> GSSMGSQSLYREIHQLISFKDVLPDKNLLPDWSSNKNPCTFDGVTCRDDKVTSIDLSSKPLNVGFSAVSSSLLSLTGLESLFLSNSHINGSVSGFKCSASLTSLDLSRNSLSGPVTTLTSLGSCSGLKFLNVSSNTLDFPGKVSGGLKLNSLEVLDLSANSISGANVVGWVLSDGCGELKHLAISGNKISGDVDVSRCVNLEFLDVSSNNFSTGIPFLGDCSALQHLDISGNKLSGDFSRAISTCTELKLLNISSNQFVGPIPPLPLKSLQYLSLAENKFTGEIPDFLSGACDTLTGLDLSGNHFYGAVPPFFGSCSLLESLALSSNNFSGELPMDTLLKMRGLKVLDLSFNEFSGELPESLTNLSASLLTLDLSSNNFSGPILPNLCQNPKNTLQELYLQNNGFTGKIPPTLSNCSELVSLHLSFNYLSGTIPSSLGSLSKLRDLKLWLNMLEGEIPQELMYVKTLETLILDFNDLTGEIPSGLSNCTNLNWISLSNNRLTGEIPKWIGRLENLAILKLSNNSFSGNIPAELGDCRSLIWLDLNTNLFNGTIPAAMFKQSGKIAANFIAGKRYVYIKNDGMKKECHGAGNLLEFQGIRSEQLNRLSTRNPCNITSRVYEGHTSPTFDNNGSMMFLDMSYNMLSGYIPKEIGSMPYLFILNLGHNDISGSIPDEVGDLRGLNILDLSSNKLDGRIPQAMSALTMLTEIDLSNNNL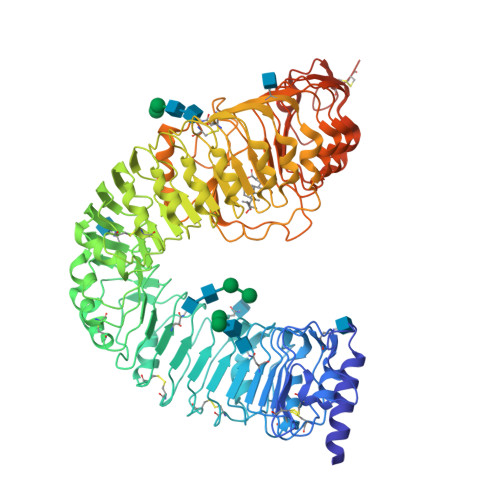SGPIPEMGQFETFPPAKFLNNPGLCGYPLPRCDPSNADGYAHHQRSHGRRLENLYFQGA>MIVSFMVAMDENRVIGKDNNLPWRLPSELQYVKKTTMGHPLIMGRKNYEAIGRPLPGRRNIIVTRNEGYHVEGCEVAHSVEEVFELCKNEEEIFIFGGAQIYDLFLPYVDKLYITKIHHAFEGDTFFPEMDMTNWKEVFVEK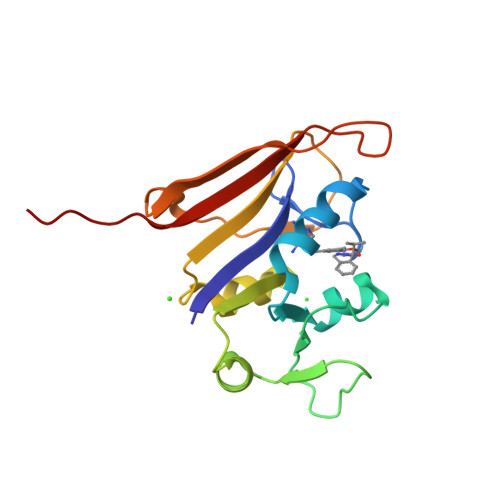GLTDEKNPYTYYYHVYEKQQLVPR[8x]> ANDTILPLNNIQGDILVGMKKQKERFVFFQVNDATSFKTALKTYVPERITSAAILISDP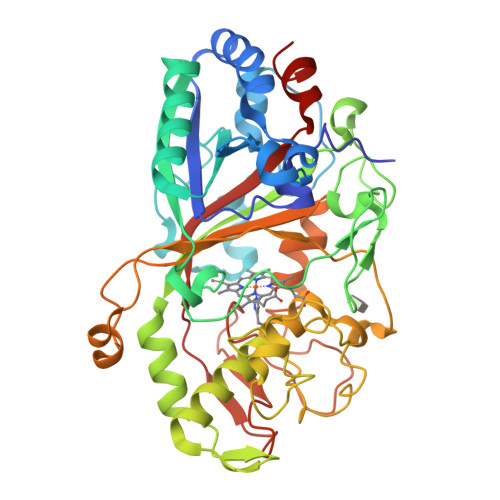SQQPLAFVNLGFSNTGLQALGITDDLGDAQFPDGQFADAANLGDDLSQWVAPFTGTTIHGVFLIGSDQDDFLDQFTDDISSTFGSSITQVQALSGSARPGDQAGHEHFGFLDGISQPSVTGWETTVFPGQAVVPPGIILTGRDGDTGTRPSWALDGSFMAFRHFQQKVPEFNAYTLANAIPANSAGNLTQQEGAEFLGARMFGRWKSGAPIDLAPTADDPALGADPQRNNNFDYSDTLTDETRCPFGAHVRKTNPRQDLGGPVDTFHAMRSSIPYGPETSDAELASGVTAQDRGLLFVEYQSIIGNGFRFQQINWANNANFPFSKPITPGIEPIIGQTTPRTVGGLDPLNQNETFTVPLFVIPKGGEYFFLPSISALTATIAA> KNDKEAAGEGPALYEDPPDQKTSPSGKPATLKICSWNVDGLRAWIKKKGLDWVKEEAPDILCLQETKCSENKLPAELQELPGLSHQYWSAPSDKEGYSGVGLLSRQCPLKVSYGIGDEEHDQEGRVIVAEFDSFVLVT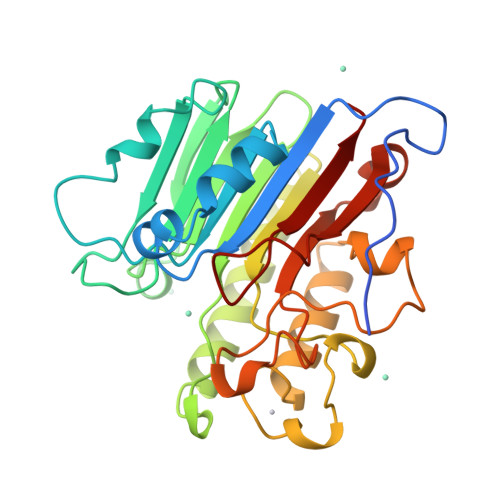AYVPNAGRGLVRLEYRQRWDEAFRKFLKGLASRKPLVLCGDLNVAHEEIDLRNPKGNKKNAGFTPQERQGFGELLQAVPLADSFRHLYPNTPYAYTFWTYMMNARSKNVGWRLDYFLLSHSLLPALCDSKIRSKALGSDHCPITLYLAL>[2x]MDFYYLPGSAPCRAVQMTAAAVGVELNLKLTNLMAGEHMKPEFLKLNPQHCIPTLVDEDGFVLWESRAIQIYLVEKYGAHDADLAERLYP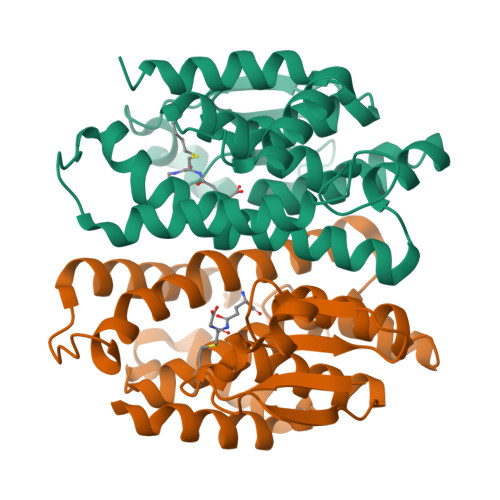SDPRRRAVVHQRLFFDVAVLYQRFAEYYEPQIFGQKVPVGDPGRLRSMEQALEFLNTFLEGEQYVAGGDDPTIADLSILATIATYEVAGYDLRRYENVQRWYERTSAIVPGADKNVEGAKVFGRYFTQK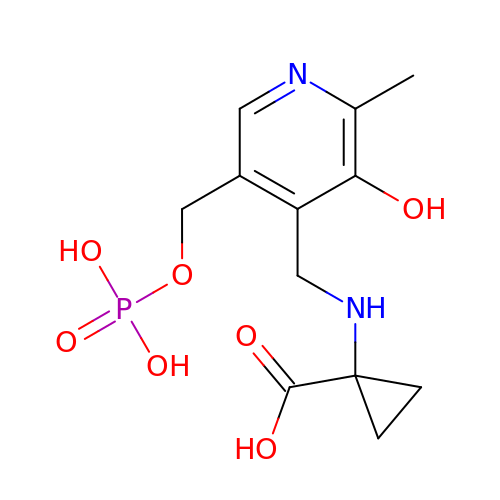N-[3-HYDROXY-2-METHYL-5-PHOSPHONOOXYMETHYL-PYRIDIN-4-Y-LMETHYL]-1-AMINO-CYCLOPROPANECARBOXYLIC ACID | C12 H17 N2 O7 P | ZMHRUAWWUAOOQN-UHFFFAOYSA-N>GSKFSRAQEKVLQKLGKAVETKDERFEQSANNFYQQQAEGHKLYKDLKNFLSAVKVMHESSKRVSETLQEIYSSEWDGHEELKAIVWNNDLLWEDYEEKLADQAVRTMEIYVAQFSEIKERIAKRGRKLVDYDSARHHLEAVQNAKKKDEAKTAKAEEEFNKA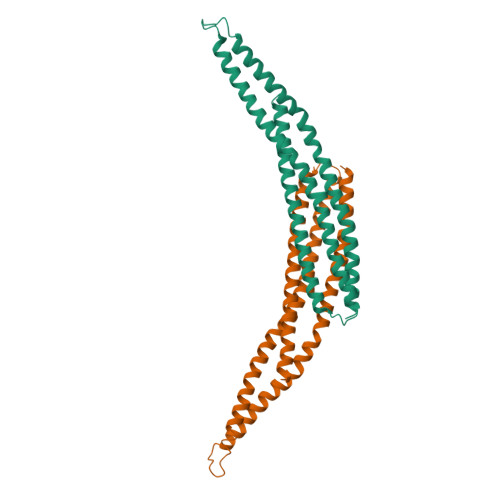QTVFEDLNQELLEELPILYNSRIGCYVTIFQNISNLRDVFYREMSKLNHNLYEVMSKL[2x]4-[(E)-({1-carboxy-2-[(3S)-2-oxo-2,3-dihydro-1H-indol-3-yl]ethan-1-id-1-yl}iminio)methyl]-2-methyl-5-[(phosphonooxy)methyl]pyridin-1-ium-3-olate 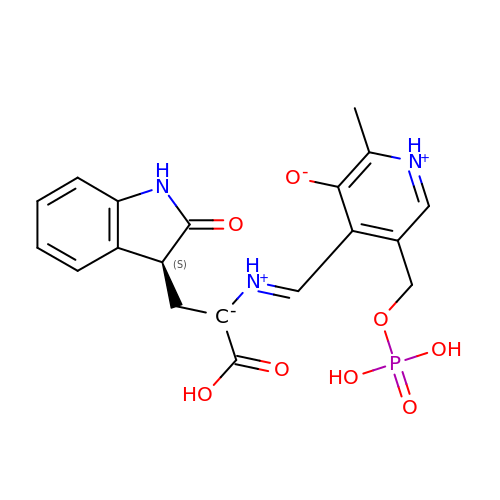| C19 H20 N3 O8 P | QWYZKAZTPCEUQJ-OOMAIKSQSA-N> MGIDINTKIFNSVAEVFQKAQGSYAGHRKHIAVLKKIQSKAVEQGYEDAFNFWFDKLVTKILPLKKNEIIDRIVKLVAAFIASLERELILAKKQNYKLTNDEEGIFSRFVDQFIRHVLRGVESPDKNVRFRVLQLLAVIMDNIGEIDESLFNLLILSLNKRIYDREPTVRIQAVFCLTKFQDEEQTEHLTELSDNEENFEATRTLVASIQNDPSAEVRRAAMLNLINDNNTRPYILERARDVNIVNRRLVYSRILKSMGRKCFDDIEPHIFDQLIEWGLEDRELSVRNACKRLIAHDWLNALDGDLIELLEKLDVSRSSVCVKAIE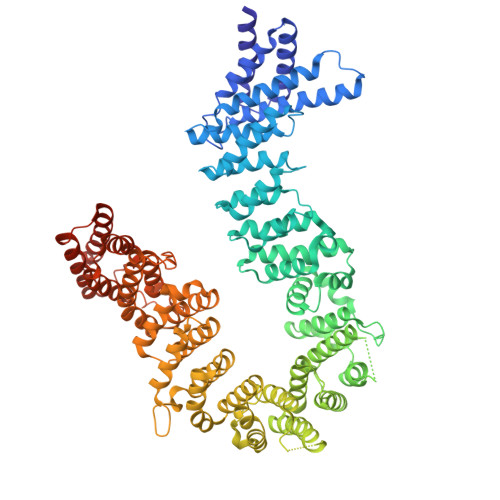ALFQSRPDILSKIKFPSIWKDFTVEIAFLFRAIYLYCLDNNITEMLEENFPEASKLSEHLNHYILLRYHHNDISNDSQSHFDYNTLEFIIEQLSIAAERYDYSDEVGRRSMLTVVRNMLALTTLSEPLIKIGIRVMKSLSINEKDFVTMAIEIINDIRDDDIEKQESESDIINNLPPEKEASSATIVLCLTRSSYMLELVNTPLTENILIASLMDTLITPAVRNTAPNIRELGVKNLGLCCLLDVKLAIDNMYILGMCVSKGNASLKYIALQVIVDIFSVHGNTVVDGEGKVDSISLHKIFYKVLKNNGLPECQVIAAEGLCKLFLADVFTDDDLFETLVLSYFSPINSSNEALVQAFAFCIPVYCFSHPAHQQRMSRTAADILLRLCVLWDDLQSSVIPEVDREAMLKPNIIFQQLLFWTDPRNLVNQTGSTKKDTVQLTFLIDVLKIYAQIEKKEIKKMIITNINAIFLSSEQDYSTLKELLEYSDDIAENDNLDNVSKNALDKLRNNLNSLIEEINERSETQTKDENNTANDQYSSILGN> MHISDEQLKRPLRDYGEALEMWSTFQTKTQALSQSLSSQLRLILTGSGIPSKRAYQILLCVDDSSSMSDDNRSTAGNLALESLVMVARALTVLEAGQIGVMGFGTDVFVAHALTDPPFTSQDAGARVLQQFTFRQDSTDMVLLLRRTIDHFREARLIQASSSRGGEDLWQLALILSDGLVQSRDHARLRPLLREAMEQRVMVVFIVMDDARSRKGHSVLELKEARFGPDGVPVIHRYLDSFPFPYYLIVHHLEDLPGALAALLRTWFAEVNSGSHHHHHH;> MKHHHHHHPMATDLGSFKANFIDSDGNQMTDVVEINFADATEKNISNLLNTLLGRDREEFT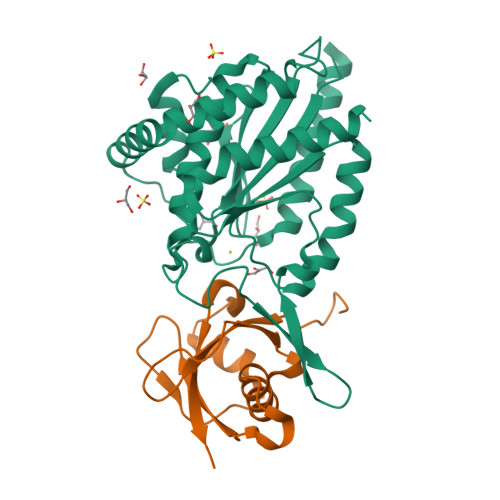PYRFRIHIPGKDLIIDQYPNDLLSLLQKHGVTNPFETTITLSAEPQA5-fluoro-2-({[(3M)-3-(1,2-oxazol-3-yl)pyridin-2-yl]amino}methyl)phenol 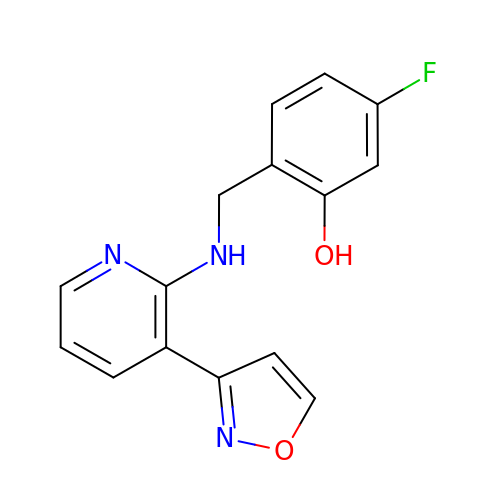| C15 H12 F N3 O2 | MUOYRIADGONWOZ-UHFFFAOYSA-N>SPNIKIFSGSSHQDLSQKIADRLGLELGKVVTKKFSNQETCVEIGESVRGEDVYIVQSGCGEINDNLMELLIMINACKIASASRVTAVIPCFPYARQDKKDKVGESRAPISAKLVANMLSVAGADHIITMDLHASQIQGFFDIPVDNLYAEPAVLKWIRENISEWRNCTIVSPDAGGAKRVTSIADRLNVDFALIHKERKKANEVDRMVLVGDVKDRVAILVDDMADTCGTICHAADKLLSAGATRVYAILTHGIFS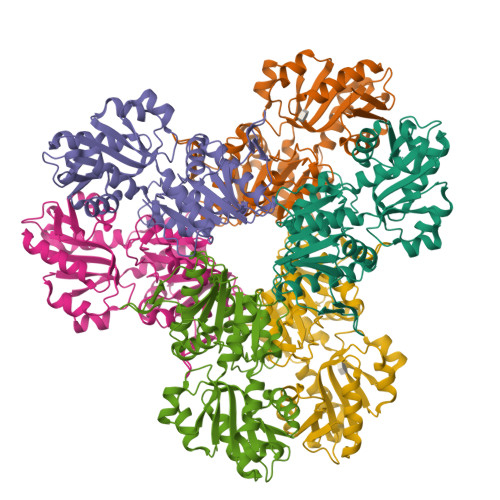GPAISRINNACFEAVVVTNTIPQEDKMKHCSKIQVIDISMILAEAIRRTHNGESVSYLFSHVPL[18x]>ALVPMVIEQTSRGERSFDIYSRLLKERVIFLTGQVEDHMANLIVAQMLFLEAENPEKDIYLYINSPGGVITAGMSIYDTMQFIKPDVSTICMGQAASMGAFLLTAGAKGKRFCLPNSRVMIHQPLGGYQGQATDIEIHAR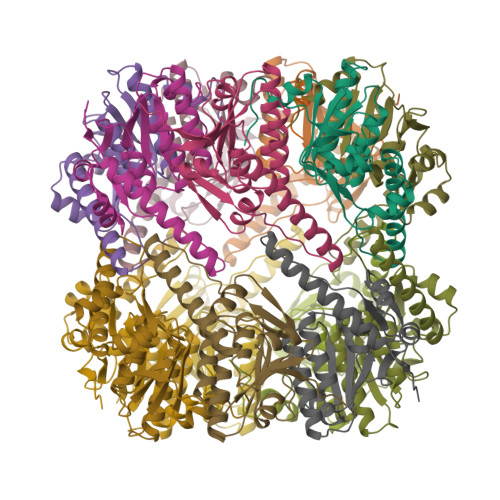EILKVKGRMNELMALHTGQSLEQIERDTERDRFLSAPEAVEYGLVDSILTHRN[14x]> NLIPTVIEQTNRGERAYDIYSRLLKDRIIMLGSAIDDNVANSIVSQLLFLAAEDPEKEISLYINSPGGSITAGMAIYDTMQFIKPKVSTICIGMAASMGAFLLAAGEKGKRYALPNS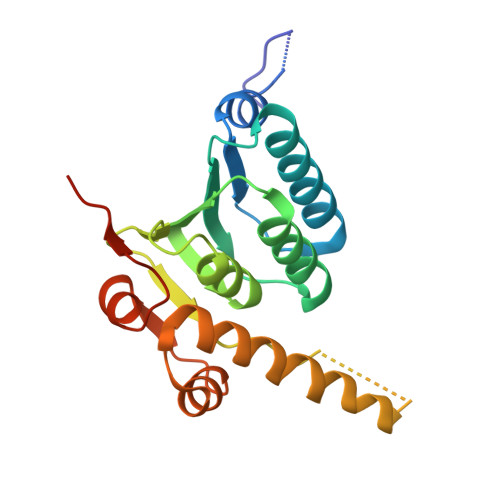EVMIHQPLGGAQGQATEIEIAAKRILLLRDKLNKVLAERTGQPLEVIERDTDRDNFKSAEEALEYGLIDKILTHLEHHHHHH>[2x]MEEPEEPADSGQSLVPVYIYSPEYVSMCDSLAKIPKRASMVHSLIEAYALHKQMRIVKPKVASMEEMATFHTDAYLQHLQKVSQEGDDDHPDSIEYGLGYDCPATEGIFDYAAAIGGATITAAQCLIDGMCKVAINWSGGWHHAKKDEASGFCYLNDAVLGILRLRRKFERILYVDLDLHHGDGVEDAFSFTSKVMTVSL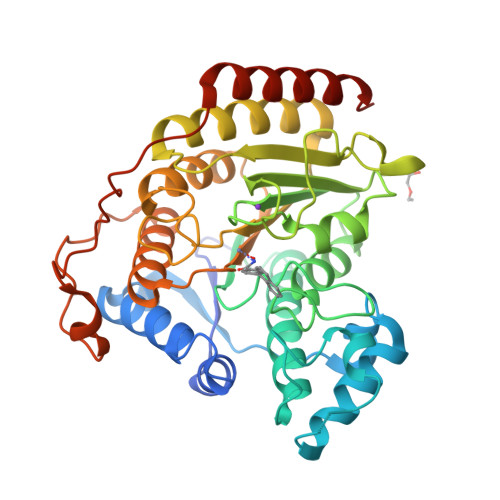HKFSPGFFPGTGDVSDVGLGKGRYYSVNVPIQDGIQDEKYYQICESVLKEVYQAFNPKAVVLQLGADTIAGDPMCSFNMTPVGIGKCLKYILQWQLATLILGGGGYNLANTARCWTYLTGVILGKTLSSEIPDHEFFTAYGPDYVLEITPSCRPDRNEPHRIQQILNYIKGNLKHVVHHHHHH>MANVLMIGFPGEGHINPSIGVMKELKSRGENITYYAVKEYKEKITALDIEFREYHDFRGDYFGKNATGDEERDFTEMLCAFLKACKDIATHIYEEVKHESYDYVIYDHHLLAGKVIANMLKLPRFSLCTTFAMNEEFAKEMMGAYMKGSLEDSPHYESYQQLAETLNADFQAEIKKPFDVFLADGDLTIVFTSRGFQPLAEQFGERYVFVGPSITERAGNNDFPFDQIDNENVLFISMGTIFNNQKQFFNQCLEVCKDFDGKVVLSIGKHIKTSELNDIPENFIVRPYVPQLEILKRASLFVTHGGMNSTSEGLYFETPLVVIPMGGDQFVVADQVEKVGAGKVIKKEELSESLLKETIQEVMNNRSYAEKAKEIGQSLKAAGGSKKAADSILEAV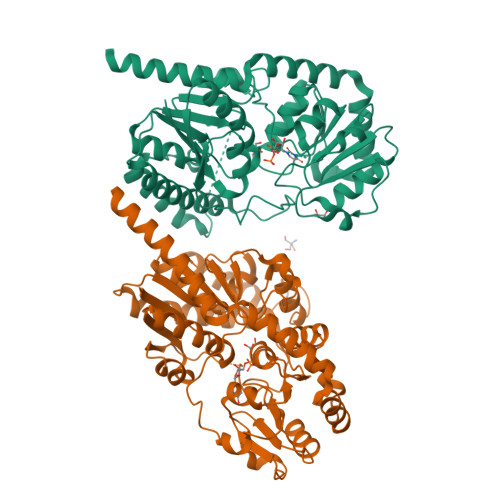KQKTQSANAALEHHHHHH[2x]>MSDDFLWFEGIAFPTMGFRSETLRKVRDEFVIRDEDVIILTYPKSGTNWLAEILCLMHSKGDAKWIQSVPIW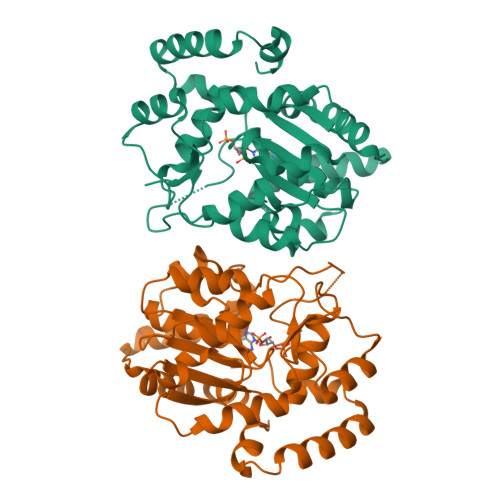ERSPWVESEIGYTALSETESPRLFSSHLPIQLFPKSFFSSKAKVIYLMRNPRDVLVSGYFFWKNMKFIKKPKSWEEYFEWFCQGTVLYGSWFDHIHGWMPMREEKNFLLLSYEELKQDTGRTIEKICQFLGKTLEPEELNLILKNSSFQSMKENKMSNYSLLSVDYVVDKAQLLRKGVSGDWKNHFTVAQAEDFDKLFQEKMADLPRKLAAALEHHHHHH[2x]> AAPNLAGAVEFSDVKTLLKEWITTISDPMEEDILQVVRYCTDLIEEKDLEKLDLV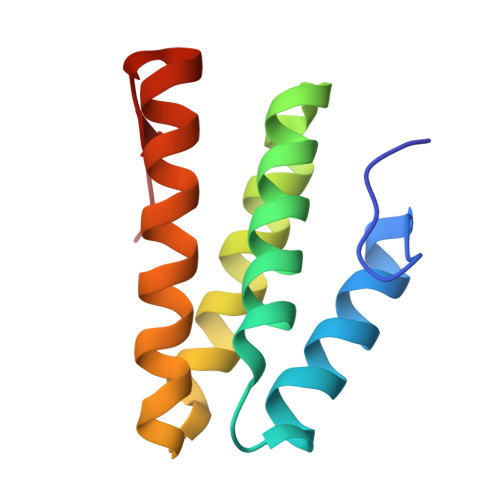IKYMKRLMQQSVESVWNMAFDFILDNVQVVLQQTYGSTLKVT>MAWSHPQFEKGHMNDANIADVVTKVLGEYGAPGAVSVAALTAKSPDGKSNSSADADVVARMVAKAIRDHAGTAQPSGNAATSSAAVSDGVFETMDAAVEAAALAQQQYLLCSMSDRARFVQGIRDVILNQDTLEKMSRMAVEETGMGNYEHKLIKNRLAGEKTPGIEDLTTDAFSGDNGLTLVEYSPFGVIGAITPTTNPTETIVCNSIGMLAAGNSVVFSPHPRARQVSLLLVRLINQKLAALGAPENLVVTVEKPSIENTNAMMAHPKVRMLVATGGPAIVKAVLSTGKKAIGAGAGNPPVVVDETANIEKAACDIVNGCSFDNNLPXVAEKEIIAVAQIADYLIFNLKKNGAYEIKDPAVLQQLQDLVLTAKGGPQTKCVGKSAVWLLSQIGISVDASIKIILMEVPREHPFVQEELMMPILPLVRVETVDDAIDLAIEVEHDNRHTAIMHSTDVRKLTKMAKLIQTTIFVKNGPSYAGLGAGGEGYSTFTIAGPTGEGLTSAKSFARRRKCVMVEALNIR[4x]

Here we systematically reconstruct a part of the metabolism of the GRM3 of Rhodopseudomonas palustris BisB18 by functionally and structurally characterizing three core enzymes, and by reconstituting the reaction sequence in vitro. Furthermore, we show that the acylating aldehyde dehydrogenase (AldDH), encoded within the GRM gene cluster, preferentially uses propionaldehyde as substrate. In summary, characterization of the GRM3 AldDH leads to a revised and detailed reaction mechanism for the ubiquitous (present in all three domains of life) family of acylating aldehyde dehydrogenases. These enzymes take part in numerous pathways including fermentations, detoxifications, other catabolic and central carbon metabolic processes.

Two different conditions were used to crystallize the AldDH with propionyl-CoA. At pH 8.1, AldDH crystallized in the monoclinic space group P 21 with one tetramer per asymmetric unit (ASU). The AldDH crystals diffracted to a resolution of 1.9 Å and the structure was solved by molecular replacement. Interestingly, we observed additional electron density around a cysteine residue in each of the putative active sites, which indicated a covalent modification. Because the enzyme was crystallized in the presence of propionyl-CoA at pH 8.1, we assumed that the corresponding cysteine residue was propionylated and modeled this residue as S-propionylcysteine. The covalent modification fit well into the electron density, to our knowledge the only acyl-enzyme thioester intermediate captured in a crystal structure of an acylating AldDH (pfam00171) to date. In three of the four active sites of the tetramer we also found coenzyme A bound in close proximity to the modified cysteine. In the fourth active site we were able to fit propionyl-CoA, which probably resulted from an additional soaking step before freezing the crystals. Interestingly, we observed that the S-propionylcysteine assumes a different rotamer conformation than the non-acylated cysteine; this has implications for the reaction mechanism. The rotation of the S-propionylcysteine also opens up space for a proton transfer relay that could serve in the deprotonation of the CoA thiol.The glycolytic enzyme fructose bisphosphate aldolase (EC 4.1.2.13) catalyzes the aldol cleavage of fructose 1,6-bisphosphate to dihydroxyacetone phosphate and glyceraldehyde 3-phosphate. It also catalyzes the reverse reaction. The hallmark of a class I aldolase is the presence of an active-site lysine residue which forms a Schiff base with the substrate. Fructose bisphosphate aldolase from E. cuniculi (EcFBPA) adopts the TIM-barrel fold typical of aldolases.

Here, we present two crystal structures of the class I fructose bisphosphate aldolase enzyme from E. cuniculi: one with the reactant bound at the active site and the other with the partial substrate mimic phosphate. For the phosphate-bound form, a data set was collected to 2.00 Å resolution. The space group was also C2221 and the unit-cell parameters were a = 121.96, b = 137.61, c = 62.23 Å. Similarly, there is clear electron density for the phosphate group in the 2.00 Å phosphate-bound structure. The purified enzyme crystallized in 90 mM Bis-Tris propane pH 6.5, 18% PEG 3350, 18 mM NaKHPO4, 10 mM urea for the phosphate-bound form and 100 mM Bis-Tris propane pH 6.5, 20% PEG 3350, 20 mM fructose 1,6-­bisphosphate for the FBP-bound form.

> GPGSMMDCDHLLRLGMTAKKILENGKGILAADETPKTLGRRFEKLGITNTEENRRKFREILFSTKGIERYIGGVILNQETFEQTSGSGVPLTELLKKKGIEIGIKLDKGLIDYKEKEKISVGLEDLDLRCKSSAFKDATFAKWRSLFYFYDGIPSEDCINENCSILAKYAIICQKNGLVPIVEPEVFLEGDYSMKRSYEVTRQILSTLMKYLNYELVYIPGVLIKASYVTSGQLSNEKYTPKKVATFTLRALLSTIPCGIPGIVFLSGGHGSEDAIGFLNAINMERGCRTWSLSFSFARALTDGVLETWRGDDSNIEEAQKILLETSFKACRGAEGKLWDQE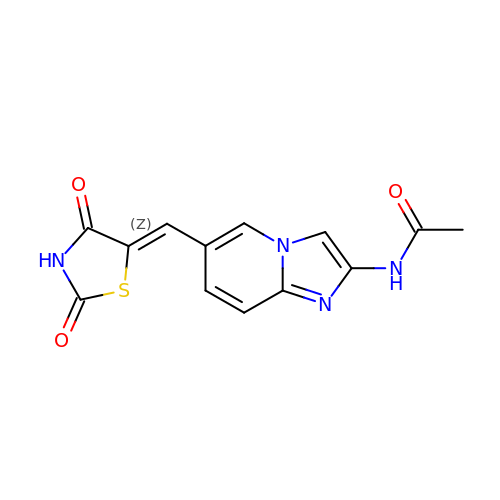N-{6-[(Z)-(2,4-dioxo-1,3-thiazolidin-5-ylidene)methyl]imidazo[1,2-a]pyridin-2-yl}acetamide | C13 H10 N4 O3 S | CCECKHDWHUIQQG-WTKPLQERSA-N> GSHMASMSHLNYLLEKIAASSKEDFPFPDDLESYLEGYVPDKNIALDTYQKIFKISSEDLEKVYKEGYHAYLDKDYAKSITVFRWLVFFNPFVSKFWFSLGASLHMSEQYSQALHAYGVTAVLRDK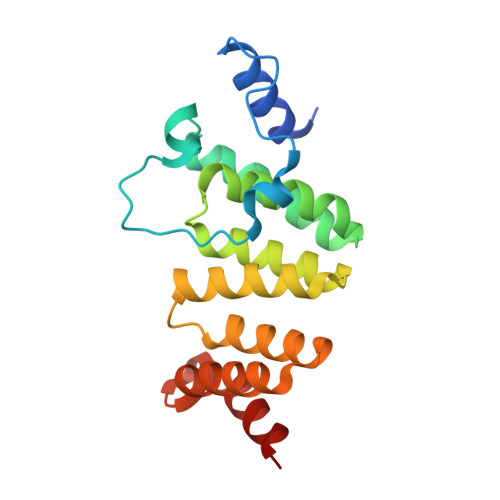DPYPHYYAYICYTLTNEHEEAEKALEMAWVRAQHKPLYNELKEEILDIRKHK> GAGTSNHDLIHSTAIIDPSAVIASDVQIGPYCIIGPQVTIGAGTKLHSHVVVGGFTRIGQNNEIFQFASVGEVCQDLKYKGEETWLEIGNNNLIREHCSLHRGTVQDNALTKIGSHNLLMVNTHIAHDCIVGDHNIFANNVGVAGHVHI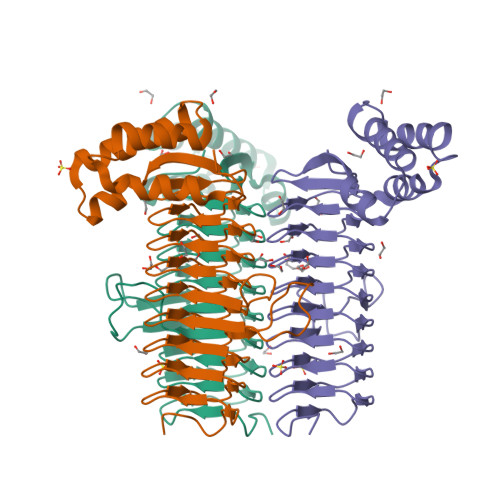GDHVIVGGNSGIHQFCKIDSYSMIGGASLILKDVPAYVMASGNPAHAFGINIEGMRRKGWSKNTIQGLREAYKLIFKSGLTSVQAIDQIKSEILPSVPEAQLLIDSLEQSERGIVR(4S)-2-(6-hydroxy-1,3-benzothiazol-2-yl)-4,5-dihydro-1,3-thiazole-4-carboxylic acid | C11 H8 N2 O3 S2 | 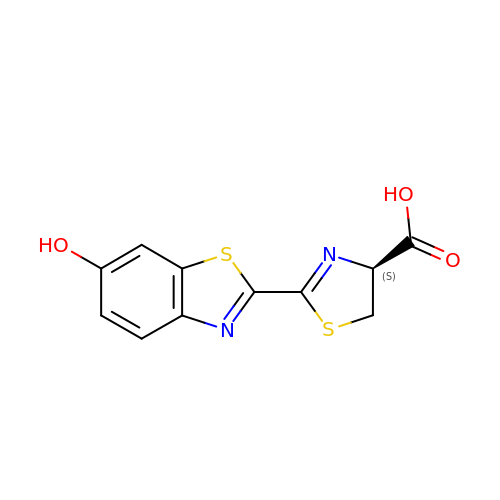BJGNCJDXODQBOB-SSDOTTSWSA-N> LIPRNALTAIVANKPFMFLIYHKPTTTVLFMGTITKGEKVIYD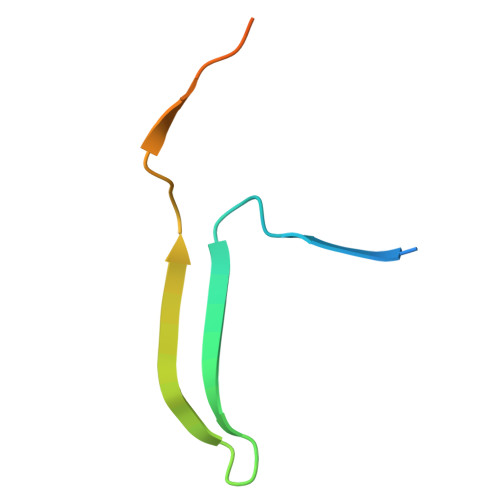TEGRDDVVSSV>[2x]SNAML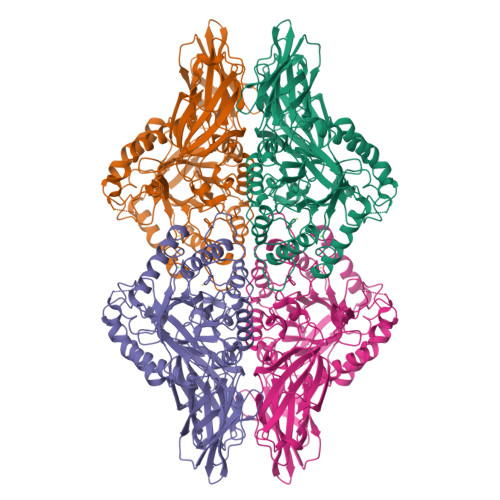YPLLTKTRNTYDLGGIWNFKLGEHNPNELLPSDEVMVIPTSFNDLMVSKEKRDYIGDFWYEKVIEVPKVSEDEEMVLRFGSVTHQAKIYVDGVLVGEHKGGFTPFEVLVPECKYNNEKIKVSICANNVLDYTTLPVGNYSEIIQEDGSIKKKVRENFDFFNYAGVHRPLKLMIRPKNHIFDITITSRLSDDLQSADLHFLVETNQKVDEVRISVFDEDNKLVGETKDSRLFLSDVHLWEVLNAYLYTARVEIFVDNQLQDVYEENFGLREIEVTNGQFLLNRKPIYFKGFGKHEDTFINGRGLNEAANLMDLNLLKDMGANSFRTSHYPYSEEMMRLADRMGVLVIDEVPAVGLFQNFNASLDLSPKDNGTWNLMQTKAAHEQAIQELVKRDKNHPSVVMWVVANEPASHEAGAHDYFEPLVKLYKDLDPQKRPVTLVNILMATPDRDQVMDLVDVVCLNRYYGWYVDHGDLTNAEVGIRKELLEWQDKFPDKPIIITEYGADTLPGLHSTWNIPYTEEFQCDFYEMSHRVFDGIPNLVGEQVWNFADFETNLMILRVQGNHKGLFSRNRQPKQVVKEFKKRWMTIPHYHNKKNSVK> FQGAMSSSIDISKINSWNKEFQSDLTHQLATTVLKNYNADDALLNKTRLQKQDNRVFNTVVSTDSTPVTNEKSSG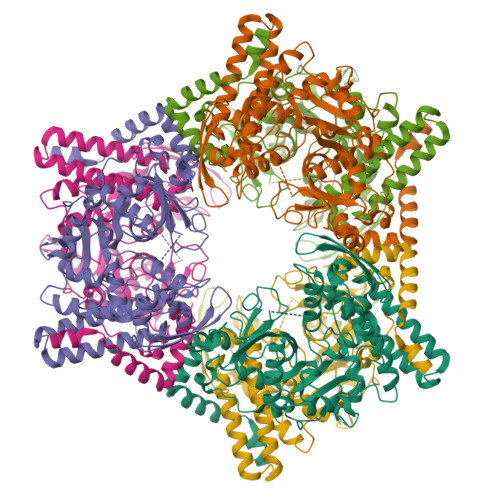RCWLFAATNQLRLNVLSELNLKEFELSQAYLFFYDKLEKANYFLDQIVSSADQDIDSRLVQYLLAAPTEDGGQYSMFLNLVKKYGLIPKDLYGDLPYSTTASRKWNSLLTTKLREFAETLRTALKERSADDSIIVTLREQMQREIFRLMSLFMDIPPVQPNEQFTWEYVDKDKKIHTIKSTPLEFASKYAKLDPSTPVSLINDPRHPYGKLIKIDRLGNVLGGDAVIYLNVDNETLSKLVVKRLQNNKAVFFGSHTPKFMDKKTGVMDIELWNYPAIGYNLPQQKASRIRYHESLMTHAMLITGCHVDETSKLPLRYRVENSWGKDSGKDGLYVMTQKYFEEYCFQIVVDINELPKELASKFTSGKEEPIVLPIWDPMGALA>[2x]MSKSRPEPVVVCLRGKSGQGKSFLANVLAQAISTHFTGAADSVWYCPPDPDHFDGYNQQAVVVMDDLGQNPDGKDFKYFAQMVSTTGFIPPMASLE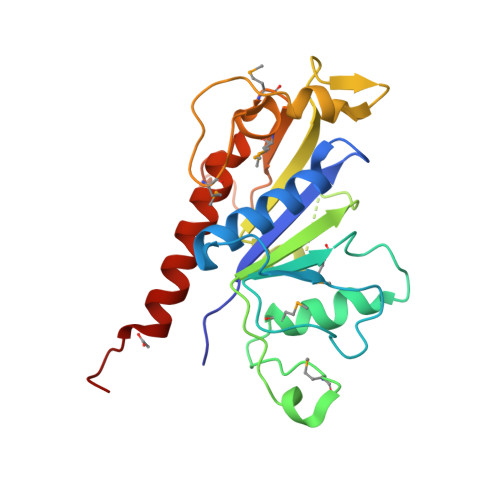DKGKPFNSKVIIATSNLYSGFTPRTMVCPDALNRRFHFDIDVSAKDGYKVNNKLDIIKALEDTHTNPVAMFQYDCALLNGMAVEMKRLQQDVFKPQPPILNVYQLVDEVIERVNLHEKVASQPIFKQ>MGSDKIHHHHHHENLYFQGMEITIFGKGNMGQAIGHNFEIAGHEVTYYGSKDQATTLGEIVIMAVPYPALAALAKQYATQLKGKIVVDITNPLNFDTWDDLVVPADSSAAQELQQQLPDSQVLKAFNTTFAATLQSGQVNGKEPTTVLVAGNDDSAKQRFTRALADSPL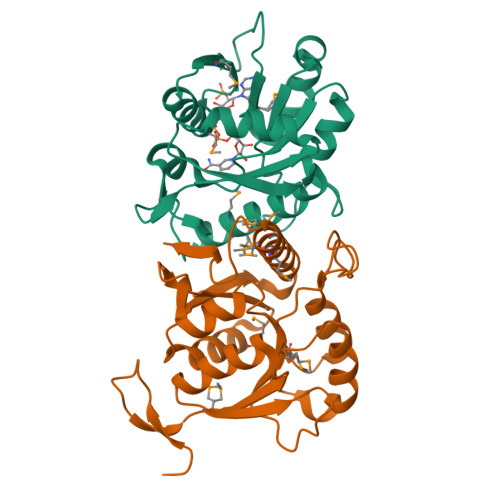EVKDAGKLKRARELEAMGFMQMTLAASEQIGWTGGFAVVK[3x]> ENNCLNAAKACNLNDTCKKYRSAYISPCTSRVSTAEVCNKRKCHKALRQFFDKVPPKHSYGMLYCSCPLG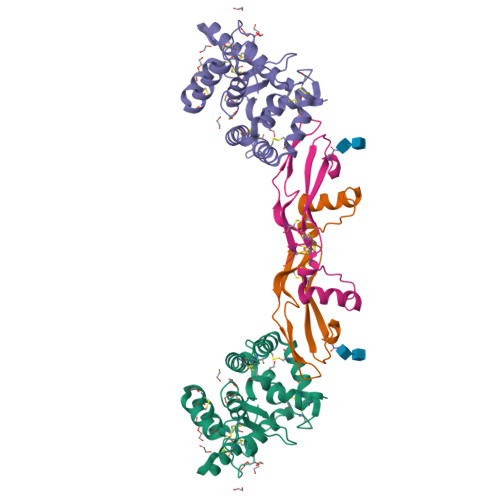DQSACSERRRQTIVPACSYEDKERPNCLTLQVSCKTNYICRSRLADFFTNCQPEPLSLSGCLKENYADCLLSYSGLIGTVMTPNYLRSPKISVSPFCDCSSSGNSKEECDRFTEFFTDNACLRNAIQAFGNGTGSEFLE;> QGRGCLLKEIHLNVTDLDLGYRTKEELIFRYCSGPCHDAETNYDKILNNLTHNKKLDKDTPSRTCCRPIAFDDDISFLDDSLEYHTLKKHSAKKCACV> MLPISMSDEGDSFLVKDSLGENKIPKNPSKVVILDLGILDTFDALKLNDKVVGVPAKNLPKYLQQFKNKPSVGGVQQVDFEAINALKPDLIIISGRQSKFYDKLKEIAPTLFVGLDNANFLSSFENNVLSVAKLYGLEKEALEKIS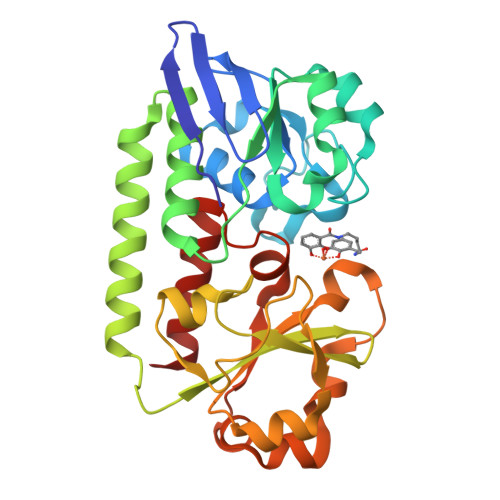DIKNEIEKAKSIVDEDKKALIILTNSNKISAFGPQSRFGIIHDVLGINAVDENIKVGTHGKSINSEFILEKNPDYIFVVDRNVILGNKERAQGILDNALVAKTKAAQNKKIIYLDPEYWYLASGNGLESLKTMILEIKNAVK>[3x]ETFTVKMGADSGLFQFEPANVTVHPGDTVKWVNNKLPPHNILFDDKQVPGASKELAD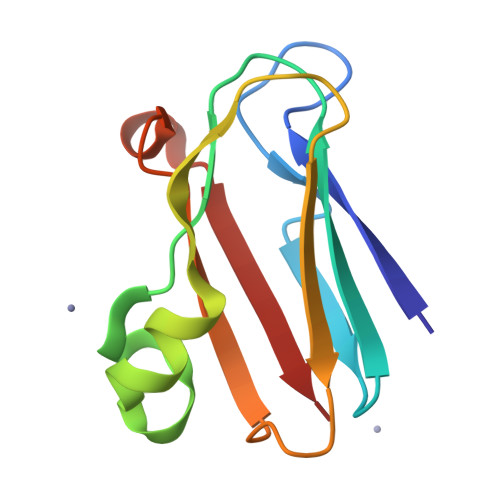KLSHSQLMFSPGESYEITFSSDFPAGTYTYYCAPHRGAGMVGKITVEG5-[2-(4-hydroxyphenyl)ethyl]benzene-1,3-diol | C14 H14 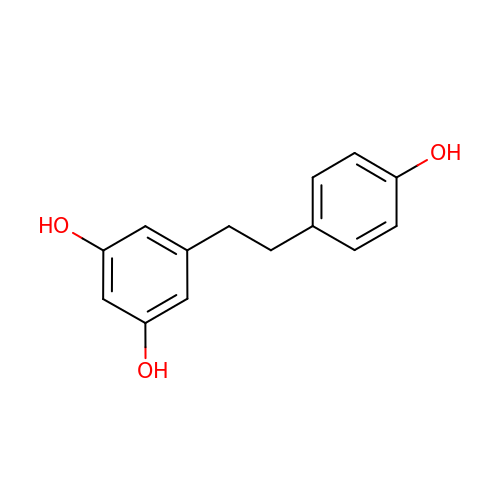O3 | HITJFUSPLYBJPE-UHFFFAOYSA-N> MPTFNPVASLKGQSVASAAQFSRADIDALIQLALDMKTHIEAGKTIDTLRGRVMTPLFFEDSSRTLSSFCAAMMRLGGSVVNFKVETSSVNKGETLQDTIRTLDSYSDVLVLRHAKEEALEQAMSVATHPIMNAGNGAGEHPTQALLDILTIHAELG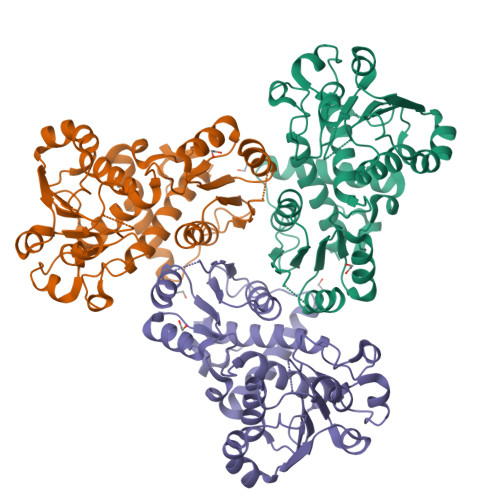AVDGIAIALIGDLKKGRTVHSLLKLLAHNFALRKVYLIAPAGLEMPAEVLEHVATDVVKRGIAIQQASGLTPEIVADCDVLYATRLQKERFVASAAGDADALTAFEASKASLLIDKARLAHAKAKMVVMHPLPRVDELSTDIDDDPRAAYFRQMRYGLFMRMAILFSVLSGHHHHHH> MVAKFQPPPEYQLTAAELKQIVDQSLSGGDLACRLLVQLFPELFSDVDFSRGCSACGFAAKRKLESLHLQLIRNYVEVYYPSVKDTAVWQAECLPQLNDFFSR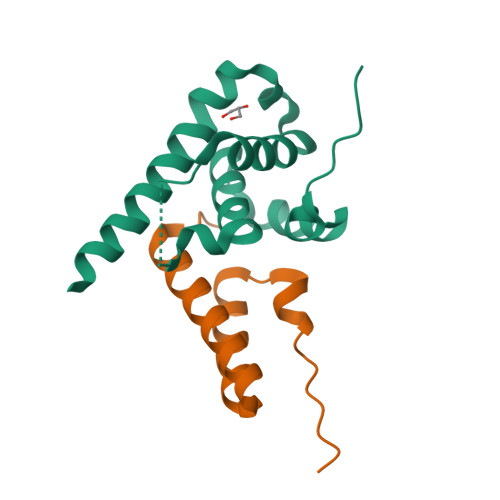FWAQREMED;> AEALSPEQAAHYLRYVKEAKEATKNGDLEEAFKLFNLAKDIFPNEKVLSRIQKIQEA> GMNNKIYFTPGPSELYPTVRQHMITALDEKIGVISHRSKKFEEVYKTASDNLKTLLELPSNYEVLFLA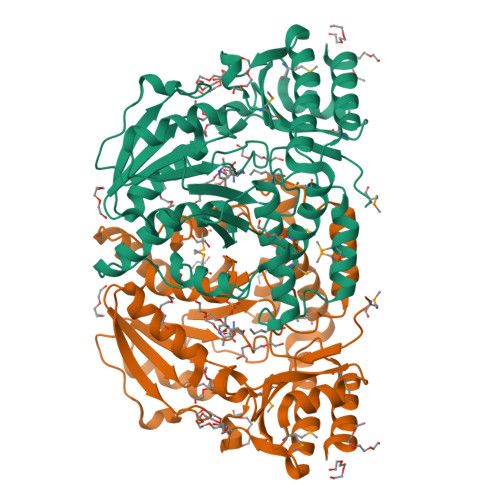SATEIWERIIQNCVEKKSFHCVNGSFSKRFYEFAGELGREAYKEEAAFGKGFYPADITVPADAEIICLTHNETSSGVSMPVEDINTFRDKNKDALIFVDAVSSLPYPKFDWTKIDSVFFSVQKCFGLPAGLGVWILNDRVIEKSKALLAKRKSIGTYHTIPSMLEKARVNQTPETPNAMNIFLLGKVTGDMLQISADGIRKQTEEKAALINTYIESSKVFSFGVEDAKLRSMTTIVANTTMLPGEINKILEPFDMAVGAGYGSKKETQIRIANFPAHSLEQVHKLVQTLKEKIG>SLSRRKPNPVIVADIRQAEGALAEIATIDRKVGEIEAQMNEAIDAAKARASQKSAPLLARRKELEDGVATFATLNKTEMFKDRKSLDLGFGTIGFRLSTQIVQMSKITKDMTLERLRQFGISEGIRIKEDVNKEAMQGWPDERLEMVGLKRRTTDAFYIEINRE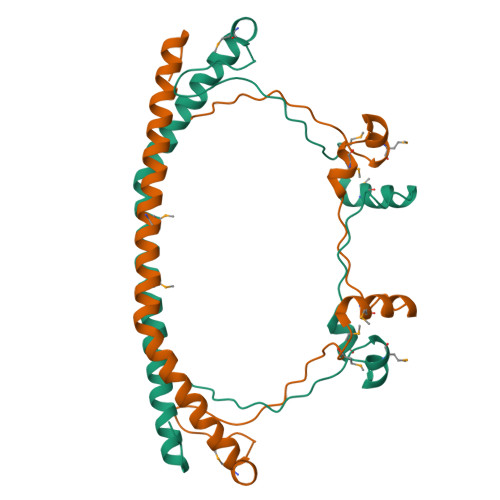EVADTAA[2x]>[2x]MAHHHHHHSLSSPYILVLYYSRHGATAEM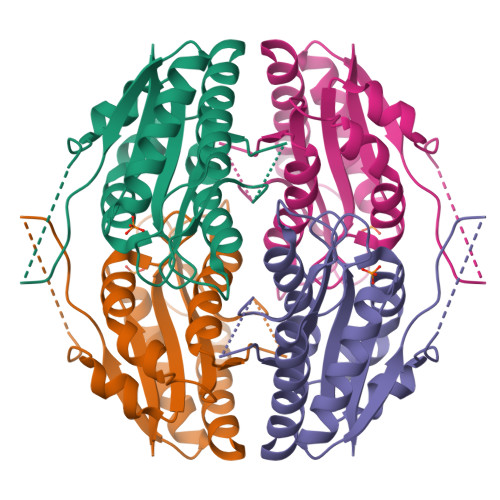ARQIARGVEQGGFEARVRTVPAVSTECEAVAPDIPAEGALYATLEDLKNCAGLALGSPTRFGNMASPLKYFLDGTSSLWLTGSLVGKPAAVFTSTASLHGGQETTQLSMLLPLLHHGMLVLGIPYSEPALLETRGGGTPYGASHFAGADGKRSLDEHELTLCRALGKRLAETAGKLEG> GSKKHSVLHLVPVNITSKADSDVTEVMWQPVLRRGRGLEAQGDIVRVWDTGIYLLYSQVLFHDVTF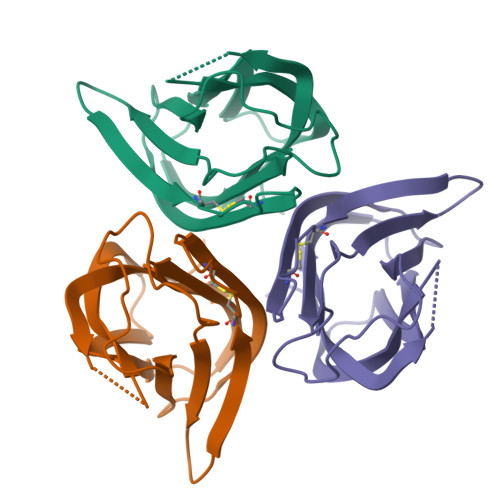TMGQVVSREGQGRRETLFRCIRSMPSDPDRAYNSCYSAGVFHLHQGDIITVKIPRANAKLSLSPHGTFLGFVKL> A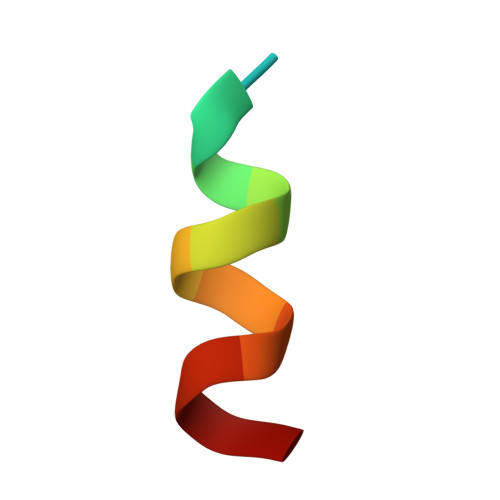TRELDELMASLS~{N}-[[1-[[3-[[4-[1-(2-azanylethanoyl)piperidin-4-yl]piperidin-1-yl]methyl]-5-[3,5-bis(chloranyl)phenyl]phenyl]methyl]piperidin-4-yl]methyl]ethanamide | C34 H47 Cl2 N5 O2 | 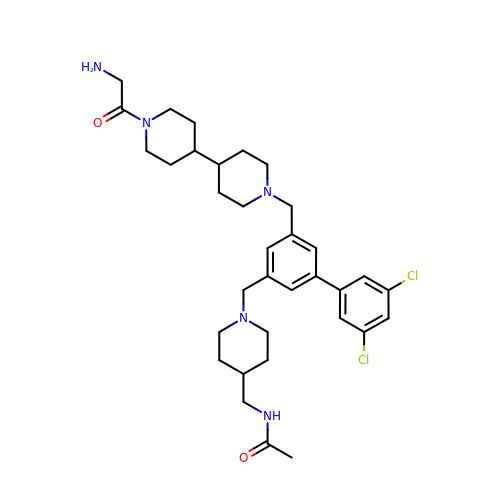OMGCBULJCZIGPC-UHFFFAOYSA-N>GSAPSRKFFVGGNWKMDGRKQSLGELIGTLNAAKVPADTEVVCAPPTAYIDFARQKLDPKIAVAAQNCYKVTNGAFTGEISPGMIKDCGATWVVLGHSERRHVFGESDELIGQKVAHALAEGLGVIACIGEKLDEREAGITEKVVFE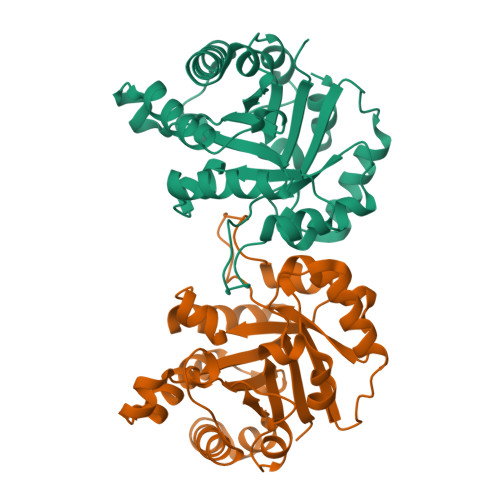QTKVIADNVKDWSKVVLAYEPVWAIGTGKTATPQQAQEVHEKLRGWLKSNVSDAVAQSTRIIYGGSVTGATCKELASQPDVDGFLVGGASLKPEFVDIINAKQ[2x]> GAMASTEKRLLKEYRAVKKELTEKRSPIHDTGIVDLHPLEDGLFRWSAVIRGPDQSPFEDALWKLEIDIPTNY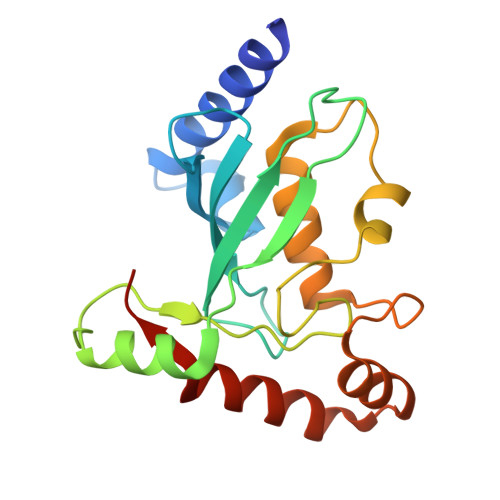PLDPPKIKFVVFGEEKIRQLQRKTSSGARKVCYKMPHPNVNFKTGEICLDILQQKWSPAWTLQSALVAIVVLLANPEPLSPLNIDMANLLKCDDTTAYKDLVHYYIAKYSAYESNDV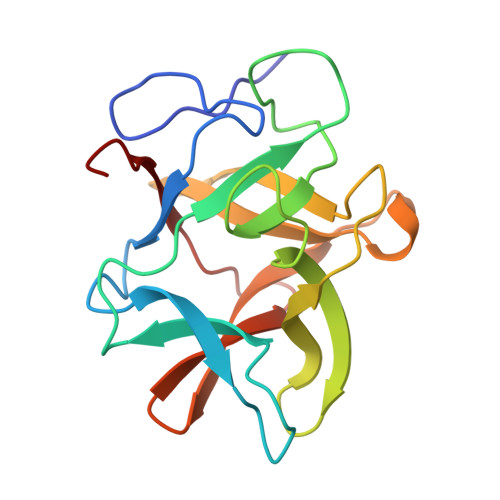> GSSVVVDTNGQPVSNGADAYYLVPVSHGHAGLALAKIGNEAEPRAVVLDPHHRPGLPVRFESPLRINIIKESYFLNIKFGPSSSDSGVWDVIQQDPIGLAVKVTDTKSLLGPFKVEKEGEGYKIVYYPERGQTGLDIGLVHRNDKYYLAVKDGEPCVFKIRKATDE1-(4-cyanophenyl)-3-(4-{[(2Z,4R)-2-imino-4-methyl-4-(2-methylpropyl)-5-oxoimidazolidin-1-yl]methyl}benzyl)urea 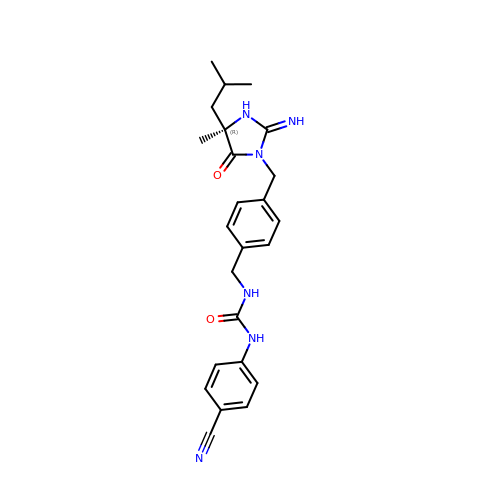| C24 H28 N6 O2 | CTKHUQYUPSHMQE-XMMPIXPASA-N> PA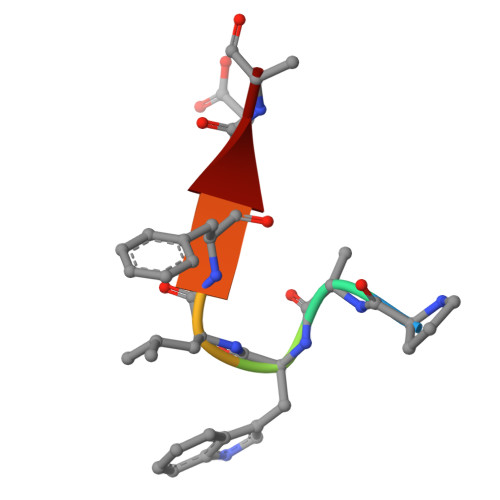WLFEA> AVSDTSGQTLNEHNELEVRYSEVLRELERRIIHLQRRINMQLQQLTLLQHNIKTQVSQILRVEVDIDVALRACKGSCARYLEYRLDKEKNLQLEKAASYIANL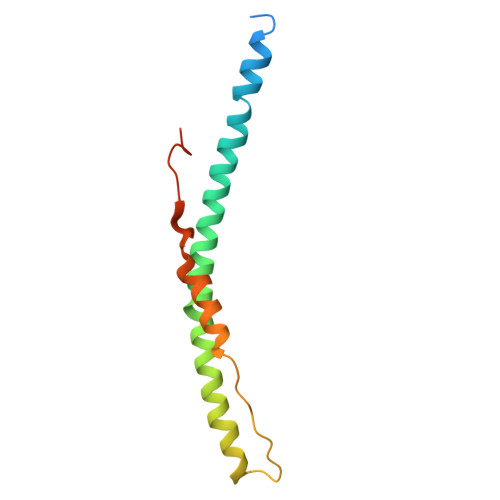KFERFEEVVVEETLNR>MGSSHHHHHHSSGRENLYFQGDIPQQLVERLQEEKRIEAQKRKERQEAHLYMQVQIVAEDQFCGHQGNDMYDEEKVKYTVFKVLKNSSLAEFVQSLSQTMGFPQDQIRLWPMQARSNGTKRPAMLDNEADGNKTMIELSDNENPWTIFLETVDPELAASGATLPKFDKDHDVMLFLKMYDPKTRSLNYCGHIYTPISCKIRDLLPVMCDRAGFIQDTSLILYEEVKPNLTERIQDYDVSLDKALDELMDGDIIVFQKDDPENDNSELPTAKEYFRDLYHRVDVIFCDKTIPNDPGFVVTLSNRMNYFQVAKTVAQRLNTDPMLLQFFKSQGYRDGPGNPLRHNYEGTLRDLLQFFKPRQPKKLYYQQLKMKITDF[2x];>GPRKCARKTRH[2x]

Ubiquitin specific protease 7 (USP7) catalyzes the deubiquitination of many cellular proteins involved in tumor suppression, neural stem cell maintenance, DNA damage and immune responses. USP7 consists of an N-terminal TRAF-like domain (NTD), a catalytic domain (CAT) and five C-terminal ubiquitin-like domains (CTD). In fact USP7 was first discovered through its strong and specific interaction with the ICP0 protein of HSV-1, leading to its original name of Herpesvirus Associated USP (HAUSP). The fact that several proteins bind to the C-terminal ubiquitin-like domains of USP7 prompted us to identify and characterize the interaction mechanism. This study shows the structural basis of interaction between the first three C-terminal ubiquitin-like domains complexed with an ICP0 peptide, revealing a protein binding pocket at Ubl2 of USP7-CTD.

The ICP0 peptide binds to a predominantly negatively charged area between 758DELMDGD764 on Ubl2. The two ICP0 lysine residues (K620 and K624) function like a pair of tongs by forming salt-bridges with two buried aspartate residues of USP7 (D762 and D764). These two lysine residues belong to the central part of the peptide (KCARKT), which is in close contact with USP7 due to a backbone-to-backbone hydrogen bond (ICP0 nitrogen-C621 with USP7 oxygen-L760). The central part of the peptide shows identical binding to both USP7 chains in the asymmetric unit and has a strong and clearly interpretable electron density. The crystal structure of all five C-terminal Ubl domains shows an extended conformation of Ubl123, matching the conformation of our Se-Ubl123 structure. A superposition of all available USP7 fragments containing Ubl123 shows two distinct orientations of Ubl3 compared to Ubl12 with a 35 degree motion and a pivot at residue H792. Closer inspection of the residues within the hinge reveals that the change in orientation is originating in the connection between Ubl2 and Ubl3, involving a change in the hydrogen bond network of residues H792, S814 and N815. Our crystallographic studies reveal a very similar orientation of the spacer helix in four crystallographically independent chains, suggesting that this helix provides a preferred orientation between CAT and Ubl12, significantly minimizing the spectrum of possible full-length conformations of USP7. The overlapping spacer helix together with the CTD now allows the generation of a nearly complete three-dimensional model of USP7, only missing some disordered N- and C-terminal residues. The resulting model of CAT-CTD is somewhat V-shaped, and intriguingly, the hinge between Ubl2 and Ubl3 (described above) affects the angle between the two arms and thereby the distance between Ubl45 and CAT. In the compact conformation of Ubl123, the distance between the catalytic domain and Ubl45 is drastically reduced from 75 Å (extended conformation) to 50 Å.> SVRRDRAPPERGGAGTSQDGTSKNWFKITIPYGRKYDKAWLLSMIQSKCSVPFTPIEFHYENTRAQFFVEDASTASALKAVNYKILDRENRRISIIINSSAPPHTILNELKPEQVEQLKLIMSKRYDGSQQALDLKGLRSDPDLVAQNIDVVLNRRSCMAATLRIIEENIPELLSLNLSNNRLYRLDDMSSIVQKAPNLKILNLSGNELKSERELDKIKGLKLEELWLDGNSLCDTFRDQSTYISAIRERFPKLLRLDGHELPPPIAFDVEAPTTLPPCKGSYFGTENLKSLVLHFLQQYYAIYDSGDRQGLLDAYHDGACCSLSIPFIPQNPARSSLAEYFKDSRNVKKLKDPTLRFRLLKHTRLNVVAFLNELPKTQHDVNSFVVDISAQTSTLLCFSVNGVFKEVDG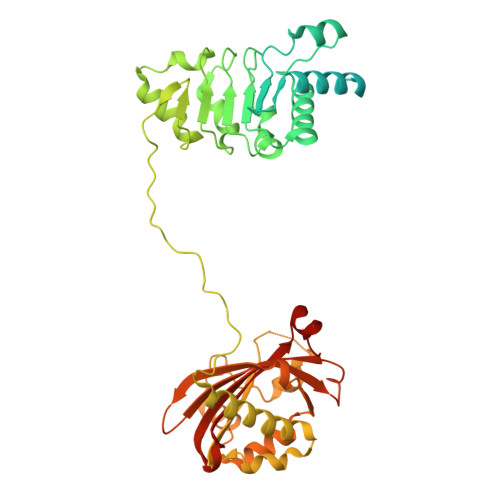KSRDSLRAFTRTFIAVPASNSGLCIVNDELFVRNASSEEIQRAFAMPAPTP>[4x]ADSGEGDFLAEGGGVRGPRVVERHQSACKDSDWPFCSDEDWNYKCPSGCRMKGLIDEVNQDFTNRINKLKNSLFEYQKNNKDSHSLTTNIMEILRGDFSSANNRDNTYNRVSEDLRSRIEVLKRKVIEKVQHIQLLQKNVRAQLVDMKRLEVDIDIKIRSCRGSCSRALAREVDLKDYEDQQKQLEQVIAKDLLPSRDRQHLPLIKMKPVPDLVPGNFKSQLQKVPPEWKALTDMPQMRMELERPGGNEITRGGSTS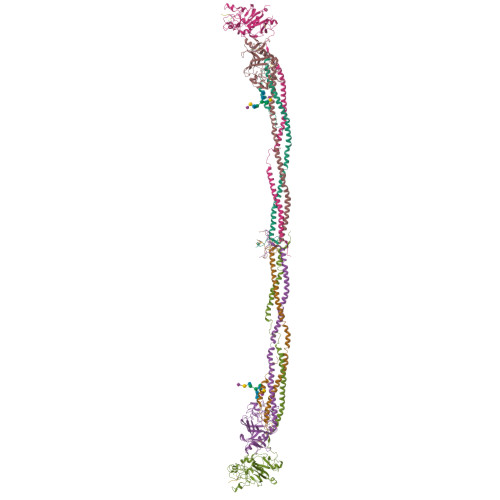YGTGSETESPRNPSSAGSWNSGSSGPGSTGNRNPGSSGTGGTATWKPGSSGPGSTGSWNSGSSGTGSTGNQNPGSPRPGSTGTWNPGSSERGSAGHWTSESSVSGSTGQWHSESGSFRPDSPGSGNARPNNPDWGTFEEVSGNVSPGTRREYHTEKLVTSKGDKELRTGKEKVTSGSTTTTRRSCSKTVTKTVIGPDGHKEVTKEVVTSEDGSDCPEAMDLGTLSGIGTLDGFRHRHPDEAAFFDTASTGKTFPGFFSPMLGEFVSETESRGSESGIFTNTKESSSHHPGIAEFPSRGKSSSYSK;>QGVNDNEEGFFSARGHRPLDKKREEAPSLRPAPPPISGGGYRARPAKAAATQKKVERKAPDAGGCLHADPDLGVLCPTGCQLQEALLQQERPIRNSVDELNNNVEAVSQTSSSSFQYMYLLKDLWQKRQKQVKDNENVVNEYSSELEKHQLYIDETVNSNIPTNLRVLRSILENLRSKIQKLESDVSAQMEYCRTPCTVSCNIPVVSGKECEEIIRKGGETSEMYLIQPDSSVKPYRVYCDMNTENGGWTVIQNRQDGSVDFGRKWDPYKQGFGNVATNTDGKNYCGLPGEYWLGNDKISQLTRMGPTELLIEMEDWKGDKVKAHYGGFTVQNEANKYQISVNKYRGTAGNALMDGASQLMGENRTMTIHNGMFFSTYDRDNDGWLTSDPRKQCSKEDGGGWWYNRCHAANPNGRYYWGGQYTWDMAKHGTDDGVVWMNWKGSWYSMRKMSMKIRPFFPQQ[4x];>YVATRDNCCILDERFGSYCPTTCGIADFLSTYQTKVDKDLQSLEDILHQVENKTSEVKQLIKAIQLTYNPDESSKPNMIDAATLKSRKMLEEIMKYEASILTHDSSIRYLQEIYNSNNQKIVNLKEKVAQLEAQCQEPCKDTVQIHDITGKDCQDIANKGAKQSGLYFIKPLKANQQFLVYCEIDGSGNGWTVFQKRLDGSVDFKKNWIQYKEGFGHLSPTGTTEFWLGNEKIHLISTQSAIPYALRVELEDWNGRTSTADYAMFKVGPEADKYRLTYAYFAGGDAGDAFDGFDFGDDPSDKFFTSHNGMQFSTWDNDNDKFEGNCAEQDGSGWWMNKCHAGHLNGVYYQGGTYSKASTPNGYDNGIIWATWKTRWYSMKKTTMKIIPFNRLTIGEGQQHHLGGAKQAGDV[4x];>GPRP[4x];>GHRP[4x]>[2x]MAKKTSSGSETPDLTVATRTGSKDLPIRNIPGNYGLPIVGPIKDRWDYFYDQGAEEFFKSRIRKYNSTVYRVNMPPGAFIAENPQVVALLDGKSFPVLFDVDKVEKKD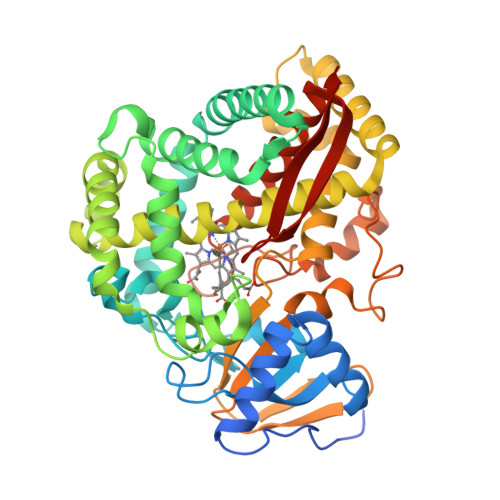LFTGTYMPSTELTGGYRILSYLDPSEPKHEKLKNLLFFLLKSSRNRIFPEFQATYSELFDSLEKELSLKGKADFGGSSDGTAFNFLARAFYGTNPADTKLKADAPGLITKWVLFNLHPLLSIGLPRVIEEPLIHTFSLPPALVKSDYQRLYEFFLESAGEILVEADKLGISREEATHNLLFATCFNTWGGMKILFPNMVKRIGRAGHQVHNRLAEEIRSVIKSNGGELTMGAIEKMELTKSVVYECLRFEPPVTAQYGRAKKDLVIESHDAAFKVKAGEMLYGYQPLATRDPKIFDRADEFVPERFVGEEGEKLLRHVLWSNGPETETPTVGNKQCAGKDFVVLVARLFVIEIFRRYDSFDIEVGTSPLGSSVNFSSLRKASFHHHH The primary mode of resistance to aminoglycoside antibiotics is through chemical modification catalyzed by aminoglycoside-modifying enzymes. Here we present the first structural and functional studies of two aminoglycoside-modifying enzymes that do not use target mimicry, AAC(3)-Ia and AAC(3)-XIa. X-ray diffraction studies reveal that these enzymes bind aminoglycoside antibiotics in a conformation where the central 2-deoxystreptamine ring is in boat conformation. Similar to other AACs, AAC(3)-Ia and AAC(3)-XIa display the GNAT superfamily fold.

In contrast, all five structures of AAC(3)-XIa contain both protomers of the physiological dimer in the asymmetric unit. The AcCoA binding pockets of both AAC(3)-Ia and AAC(3)-XIa have a similar tunnel-like conformation that extends to the aminoglycoside binding pocket, and our structures show that the overall binding of the CoA molecules is conserved across all of the structures. In all our structures, the highest concentration of hydrogen bond interactions between enzyme and CoA occurred in the pyrophosphate moiety. The greatest difference between the coenzyme-bound structures of both AAC(3)-Ia and AAC(3)-XIa occurs in the positioning of the adenosine moiety. In the AAC(3)-Ia structures, there is a shift of around 90°, and in the AAC(3)-XIa binary structure with AcCoA, we see a rotation of the ADP moiety of around 180°. The flipping of this group can be attributed to the solvent-exposed nature of the adenine binding pockets of AAC(3)-Ia and AAC(3)-XIa.

>MTTTNEIRVAEVADAGVVAKLLRDFNTEFDTPVPEGLEERFAQIIAHDDAFVLLAGDIGFAYVTLRPSPYYDGPVAMLDELYVAPAHRNRGVGTALLQRVFEEIRKHSAGELQINVDEVDTDARRFYERHGLTNIEQGSRMLLYIREL[2x]6-{[(3R,4R)-4-(2-{[2-(3-chlorophenyl)-2,2-difluoroethyl]amino}ethoxy)pyrrolidin-3-yl]methyl}-4-methylpyridin-2-amine 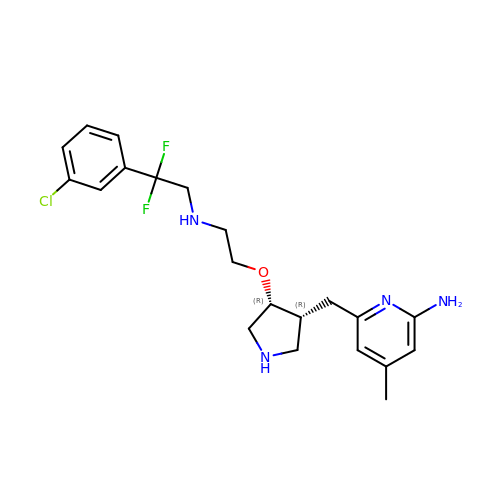| C21 H27 Cl F2 N4 O | UAYPWJGHCQAPDA-BEFAXECRSA-N NDM-1 belongs to the B1 subclass of MBLs that requires a dinuclear metal center for full catalytic activity. Zn1 is ligated to three histidine residues, H120, H122, and H189, while Zn2 is coordinated with D124, C208, and H250. To address whether carbapenems undergo pyrroline tautomerization during hydrolysis and whether diverse protonation mechanisms exist for different β-lactams, we conduct a combined investigation on NDM-1-catalyzed hydrolysis of imipenem and meropenem using X-ray crystallography and NMR spectrometry. Our data presented here revealed informative details of the reaction including (i) double-bond tautomerization in the pyrroline ring following the cleavage of the lactam amide bond; (ii) three derivatives presumably representing EI1, EI2, and EP; (iii) absence of the bridging water molecule attributed to steric hindrance from the newly formed carboxylate that is forced to take a distinctive orientation resulting from the trans configuration of the β-lactam ring in carbapenems; and (iv) exclusive stereoselective protonation of the carbanionic intermediates.

Six imipenem-bound and five meropenem-bound structures were determined by molecular replacement and refined at resolutions from 1.80 to 2.32 Å. We first modeled hydrolyzed imipenem or meropenem in the Δ2 isoform in all crystals and found that the ligands could be well fitted in density in some structures with good planarity remaining among C1, C2, C3 and the sulfur atom bonded to the R2 side chain during refinement. We finally modeled Δ2 (EI1) in one imipenem- and three meropenem-bound structures and Δ1 (EI2 or EP) in five imipenem- and two meropenem-bound structures. In four imipenem- and all five meropenem-bound structures determined in this study, the carbapenem intermediates present in either Δ2 (EI1) or Δ1 (EI2) bind the dinuclear metal center in a consensus manner with hydrolyzed penicillins or cephalosporins revealed in NDM-1 strucutures. The newly formed C6-carboxylate contacts Zn1, while the lactam nitrogen (N4) and C3-carboxylate interact with Zn2. The sulfur-bonded pyrrolidine ring in meropenem was also well defined in density, but the hydrophilic formimidamide group in imipenem was rather mobile, as indicated by higher B-factors or even the absence of visible density. The crystallographic entrapment of both Δ2 and Δ1 isomers sufficiently demonstrates that hydrolysis proceeds via an open-ring derivative with a negative charge delocalized over a conjugated π-system covering C2 and N4, which is dynamically stabilized at the active site of NDM-1. A tentative equilibrium between the two intermediates, EI1 and EI2, is thus established before protonation occurs. Owing to the lack of the bridging water that may serve as an ideal proton donor, protonation at the lactam nitrogen (N4) seems to be impossible.

>[8x]GEIRPTIGQQMETGDQRFGDLVFRQLAPNVWQHTSYLDMPGFGAVASNGLIVRDGGRVLVVDTAWTDDQTAQILNWIKQEINLPVALAVVTHAHQDKMGGMDALHAAGIATYANALSNQLAPQEGMVAAQHSLTFAANGWVEPATAPNFGPLKVFYPGPGHTSDNITVGIDGTDIAFGGCLIKDSKAKSLGNLGDADTEHYAASARAFGAAFPKASMIVMSHSAPDSRAAITHTARMADKLR The principal constituent of the protein deposits is one of the most abundant proteins in the extracellular matrix (ECM) of the human cornea, transforming growth factor-β–induced protein (TGFBIp). The function of corneal TGFBIp is elusive, but its ability to bind both integrins and ECM molecules indicates a role in cell adhesion. TGFBIp consists of an N-terminal CROPT domain followed by four fasciclin 1 (FAS1) domains (FAS1-1, FAS1-2, FAS1-3, and FAS1-4). The X-ray crystal structure of wildtype TGFBIp reveals an elongated banana-shaped molecule with the five domains arranged like pearls on a curved string.

Among the most frequent pathogenic mutations are R124H and R555W, both associated with granular corneal dystrophy (GCD) characterized by the early-onset formation of amorphous aggregates. A striking feature found in both the R124H and R555W structures and involving their mutated residues is a crystal packing interface between the FAS1-1 and FAS1-4 domains of different TGFBIp molecules, where residue 124 interacts with residue 555 in a second TGFBIp molecule (i.e., His124 and Arg555 in R124H, Arg124 and Trp555 in R555W). In the much more hydrophobic R555W interface, there are no water molecules close to Trp555. The interface is organized around the Trp555 side chain, and similarly to the R124H interface, the tryptophan indole ring is surrounded by a hydrophobic shell of side chains contributed by Phe547, Leu550, Leu558, Leu559, Leu120, Y121, Val163, and Leu167. A crucial interaction sealing the pocket around Trp555 is made by Arg124 from the second TGFBIp molecule, as its guanidinium group stacks with the tryptophan indole ring in a cation–π interaction. In addition, the Arg124 side chain further stabilizes the intermolecular interaction through hydrogen bonds with the main-chain carbonyl groups of Leu550 and Phe547. The FAS1-1:FAS1-4 interface in the R555W structure is significantly more hydrophobic than in the R124H structure, with a ΔiG p-value of 0.11 and 0.40, respectively. This R555W FAS1-1:FAS1-4 interface is also by far the most hydrophobic in all the four TGFBIp crystal structures determined to date and has a calculated ΔiG of −9 kcal/mol, which is also the most favorable value of all the intermolecular contacts present in these structures. The Arg124 and Arg555 residues in wildtype TGFBIp do not permit this intermolecular interface due to size and electrostatic repulsion between the two arginines.

> GPNVCAVQKVIGTNRKYFTNCKQWYQRKICGKSTVISYECCPGYEKVPGEKGCPAALPLSNLYETLGVVGSTTTQLYTDRTEKLRPEMEGPGSFTIFAPSNEAWASLPAEVLDSLVSNVNIELLNALRYHMVGRRVLTDELKHGMTLTSMYQNSNIQIHHYPNGIVTVNCARLLKADHHATNGVVHLIDKVISTITNNIQQIIEIEDTFETLRAAVAASGLNTMLEGNGQYTLLAPTNEAFEKIPSETLNRILGDPEALRDLLNNHILKSAMCAEAIVAGLSVETLEGTTLEVGCSGDMLTINGKAIISNKDILATNGVIHYIDELLIPDSAKTLFELAAESDVSTAIDLFRQAGLGNHLSGSERLTLLAPLNSVFKDGTPPIDAHTRNLLRNHIIKDQLASKYLYHGQTLETLGGKKLRVFVYRNSLCIENSCIAAHDKRGRYGTLFTMDRVLTPPMGTVMDVLKGDNRFSMLVAAIQSAGLTETLNREGVYTVFAPTNEAFRALPPREWSRLLGDAKELANILKYHIGDEILVSGGIGALVRLKSLQGDKLEVSLKNNVVSVNKEPVAEPDIMATNGVVHVITNVLHHHHHH The Tn1549 conjugative transposon propagates resistance to the antibiotic vancomycin used for severe drug-resistant infections. The DNA cleavage and joining reactions required for CTn transposition are carried out by a transposase enzyme called integrase (Int). Most known CTns, including the Tn916-like family, have Y-transposases that use a conserved tyrosine residue to attack a phosphorous atom in the DNA backbone. Int contains 3 functional domains: an arm-binding domain (AB), a core DNA binding domain (CB), and a catalytic domain (CAT).

We obtained crystals of Int82N bound to a 44 bp double-stranded DNA (dsDNA) oligonucleotide mimicking the CI. The DNA (named CI5) represents a sequence from previous in vivo studies in Clostridium and contains the conserved left and right 11 bp long AT-rich imperfect inverted repeats (IRL and IRR) that mark the ends of Tn1549, connected by a 5 bp homoduplex crossover region (atagc) (Domingo et al., 2005) as in the transposon integration substrate in the recipient cell. (A) Close-up of the active site in the wild-type Int82N-CI5 complex structure shows the same architecture as in the R225K mutant. As before, Y379 points toward the DNA at the phosphate of T-1/T-1’ (at 5.2-5.8 Å distance). R225 forms a hydrogen bond with the scissile phosphate (T-1/T-1’). The structures superpose with RMSD of 0.5020 Å for Cα atoms in Molecule A.

>[2x]SMTVCQLYAKQIRHRGNVKHNTKLGRERLMRILEQDRLGSCPIDSVKLSDAKEWALRMKEKGLSYKTINNDKRSLKAAFYTAIQDDCIRKNPFDFQLSDVLDDDTEPKVPLTPAQEESFLSFIQGDKVYQKHYDAIVILLGTGLRISELCGLTDKDLDFENRVIIVSHQLLRNTGVGYYIDEPKTQSGVRKIPMNEEVYQAFQRVIKNRKGAKPFIIDGYANFLFLKQNGYPMTAVDYGGMFGRLVKKYNKSHEEALPKTTTPHAMRHTFCTRLANAGMNPKALQYIMGHSNITMTLNYYAHATFDSARAEMERLAA> MGSSHHHHHHMPFTIDSARGIFPNTLAADVVPATIARFSQLNAEDQLALIWFAYLEMGKTLTIAAPGAASMQLAENALKEIQAMGPLQQTQAMCDLANRADTPLCRTYASWSPNIKLGFWYRLGELMEQGFVAPIPAGYQLSANANAVLATIQGLESGQQITVLRNAVVDMGFTAGKDGKRIAEPVVPPQDTASRTKVSIEGVTNATVLNYMDNLNANDFDTLIELFTSDGALQPPFQRPIVGKENVLRFFREECQNLKLIPERGVTEPAEDGFTQIKVTGKVQTPWFGGNVGMNIAWRFLLNPEGKIFFVAIDLLASPKELLNFAR

Orange Carotenoid protein (OCP) is the only known photoreceptor which uses carotenoid for its activation. It is found exclusively in cyanobacteria, where it functions to control light-harvesting of the photosynthetic machinery. In the active state, following OCPR (red state) binding to the cyanobacterial light-harvesting antenna, the keto-carotenoid dissipates excess absorbed light energy through non-photochemical quenching (NPQ), a vital process for cyanobacterial survival in turbulent waters.

In contrast to a previous crystallographic investigation of OCP photoactivation, we observe that the absorbance spectra of OCPO in solution and in crystals are nearly identical, thereby providing evidence for the same electronic structure of the carotenoid in both crystals and solution. The data furthermore supports identification of glycerol, acetate, the Cl− ion and 401 water molecules in the crystal structure. The location of Cl− in this study was confirmed by long-wavelength X-ray crystallography. Cl− is resolved in the CTD, where it coordinates four water molecules through ion–dipole interactions at distances of 3.0–3.2 Å (HOH16, HOH23, and HOH46) and 4.0 Å (HOH41). The closest CAN carbon is C12, located at 4.1 Å distance from the Cl− ion in the CTD. Three amino acids (L248, T275, and P276) are within 4 Å distance from Cl−. Tyrosine Y44 and tryptophan W110 are located in closest proximity (4Å) to the C6’-C7’ = C8’-C9’ moiety in the hydrophobic pocket which also contains the β2-ring of the carotenoid. Together with W41, residues Y44 and W110 interact with the carotenoid β2-ring through π-π stacking.> SSPSSPLYFEGPSYGIRVSVGSNKQEQQVVLDTGSSDFWVVDSSASCQKGNCKQYGTFDPHSSTSFKSLGSSFSIGYGDKSSSIGTWGQDTIYLGGTSITNQRFADVTSTSVNQGILGVGRVETESANPPYDNVPITLKKQGKIKTNAYSLYLNSPGAATGTIIFGGVDNAKYSGKLIEEPLVSDRYLAVNLKSLNYNGDNSNAGFGVVVDSGTTISYLPDSIV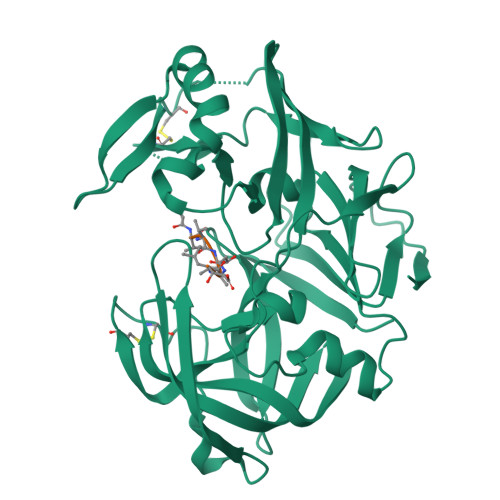DDLANKVGAYLEPVGLGNELYFIDCNANPQGSASFTFDNGAKITVPLSEFVLQSTANACVWGLQSSDRQNVPPILGDNFLRHAYVVFNLDKETVSLAQVKYTSASSVSAI>MGSSHHHHHHSQDPNSNQAQELNH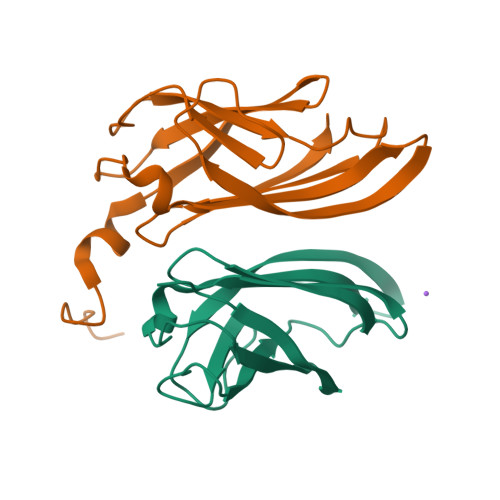ELELEQLETKITVSSVSLTGSTLNVVLENNGSTNLYDFQGFSVIVQYYANISNISTFNLSLYNYTKNSNPSPYYWTINTPLLAPGSQATLTIILPYPPYPNTQATVVIVTNYGPSVIWRGSL[2x]> GPQLTIEVLVTVDGVNFRTVVLNNKNTYRSQLGCVFFNGADISDTIPDEKQNGHSLYLADNLTADETKALKELYGPVDPTFLHRFYSLKAAVHGWKMVVCDKVRSLKLSDNNCYLNAVIMTLDLLKDIKFVIPALQHAFMKHKGGDSTDFIALIMAYGNCTFGAPDDASRLLHTVLAKAELCCSARMVWREWCNVCGIKDVVLQGLKACCYVGVQTVEDLRARMTYVCQCGGERHRQLVEHTTPWLLLSGTPNEKLVTTSTAPDFVAFNVFQGIETAVGHYVHARLKGGL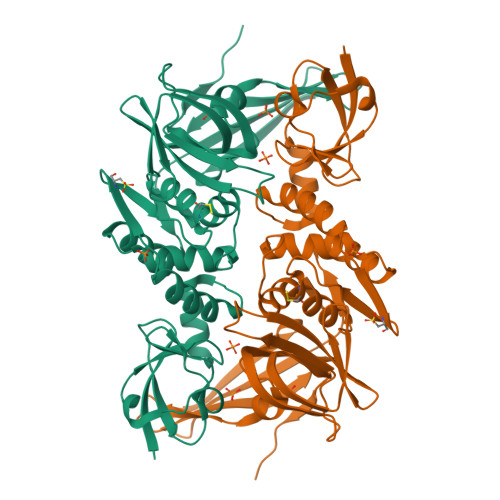ILKFDSGTVSKTSDWKCKVTDVLFPGQKYSSDCN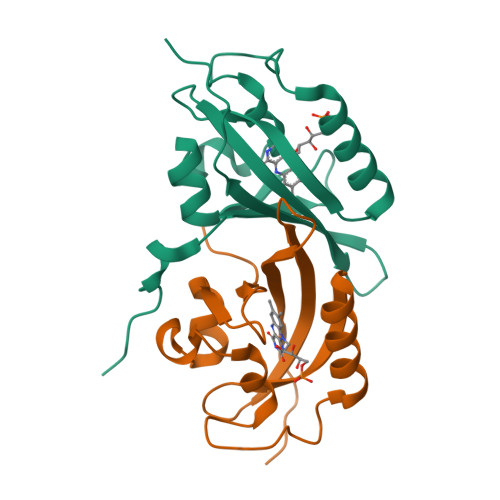>[4x]GGPIPYPVGNLLHTAPCGFVVTDAVEPDQPIIYVNTVFEMVTGYRAEEVLGGNCRFLQCRGPFAKRRHPLVDSMVVSEIRKCIDEGIEFQGELLNFRKDGSPLMNRLRLTPIYGDDDTITHIIGIQFFIETDIDLGP> MQ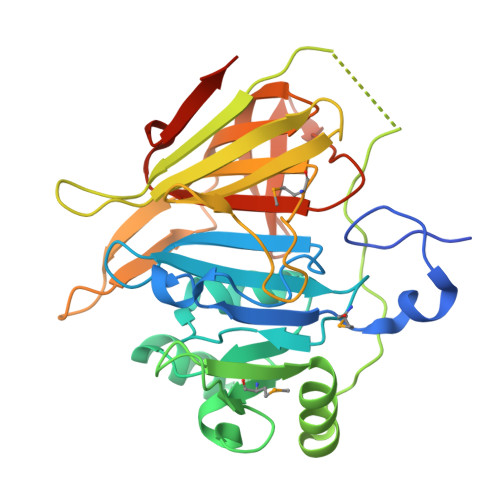QKDAVPDTAKKLKAPLTGLKTEQKVTERRPVAVVVNNHPKARPQSGLSKADIVIEALAEGQITRFLAIFQSQMPETVGPVRSAREYFVTLSNGFDSIFVHHGWSPGAKKQLESGAADYMNGLDFDGSLFWRADFSKPPHNSYTSYDYIKKAAEQKGYKLKQETNPLLFQTSDAKPANESYNVRVDYGTNNVTNLVEYNYDKKAEFYTRSSDGVITTDRETGKPVAMQNIFIVEASHHIIDQDGRRDIDLESGGKGLLFQHGNVIETDWKQVNGRIVPVKDGKWLPFVPGKTWINIVPDLDAASISKGEGVLEHHHHHH> AFTLADRVTEEMLADKAALVVEVVEENYHDAPIVGIAVVNEHGRFFLRPETALADPQFVAWLGDETKKKSMFDSKRAAVALKWKGIELCGVSFDLLLAAYLLDPAQGVDDVAAAAKMKQYEAVRPDEAVYGKGAKRAVPDEPVLAEHLVRKAAAIWALERPFLDELRRNEQDRLLVELEQPLSSILAEMEFAGVKVDTKRLEQMGEELAEQLRTVEQRIYELAGQEFNINSPKQLGVILFEKLQLPVLKKTKTGYSTSADVLEKLAPYHEIVENILHYRQLGKLQSTYIEGLLKVVRPDTKKVH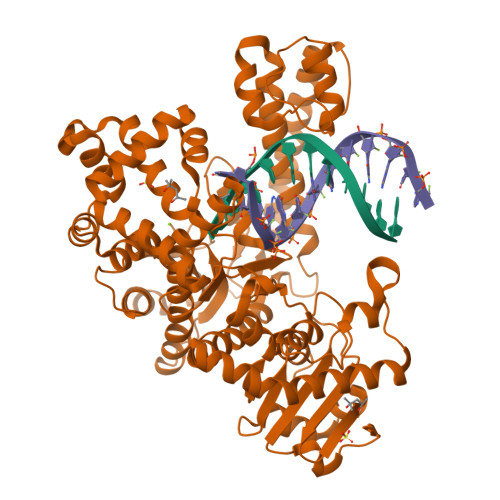TIFNQALTQTGRLSSTEPNLQNIPIRLEEGRKIRQAFVPSESDWLIFAADYSQIELRVLAHIAEDDNLMEAFRRDLDIHTKTAMDIFQVSEDEVTPNMRRQAKAVNFGIVYGISDYGLAQNLNISRKEAAEFIERYFESFPGVKRYMENIVQEAKQKGYVTTLLHRRRYLPDITSRNFNVRSFAERMAMNTPIQGSAADIIKKAMIDLNARLKEERLQARLLLQVHDELILEAPKEEMERLCRLVPEVMEQAVTLRVPLKVDYHYGSTWYDAK>TAGGGT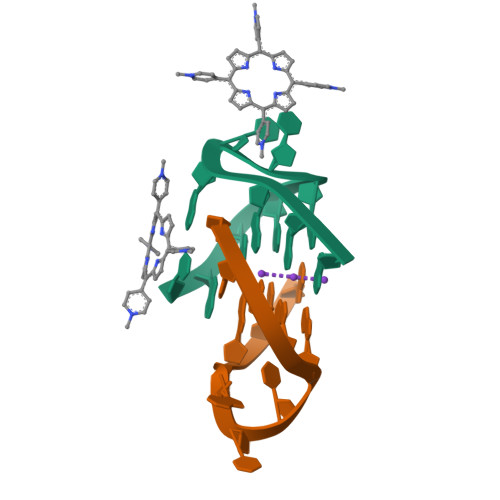TAGGG[2x]> MNHKVHHHHHHIEGRHMNATVETTQHDVEGTGAAGATAMLFPGMGPAAFSDVGRFMVTNRYTRELLAEADDTLGYSLVDRFRQAEGDYSEYAQIAFLVNCVALARWAEQTMDLTPRICAGASFGEKSVAAYSGALTFADAVRMTAGLARCMDEYFRTEHLGVVTHSFVRAPRERLDEILAELDERGEWHEISCHIDHDFFMLTLHERNSVWLEGRLRSVGAMPLYAMRPPMHAAAFGGLRDKAEEEVIAPLTFHDPTLPVVADQDGKVLTTGDEVRTMLL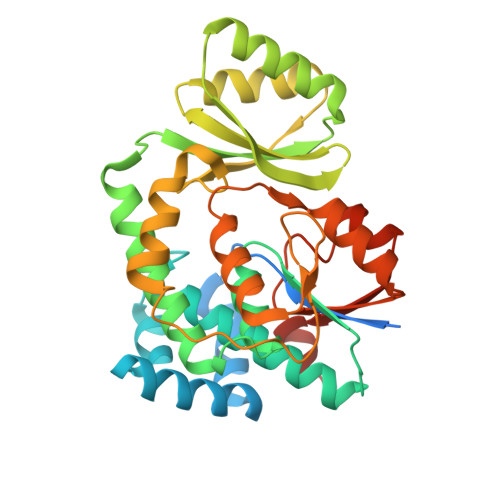ECFVRPLRWPDVISSLQDQGVTRVCVAGPDSLFGRVGTTTRAFEVIAATPRLALQPRARTTSR>SPNIKIFSGSSHQDLSQKIADRLGLELGKVVTKKFSNQETCVEIGESVRGED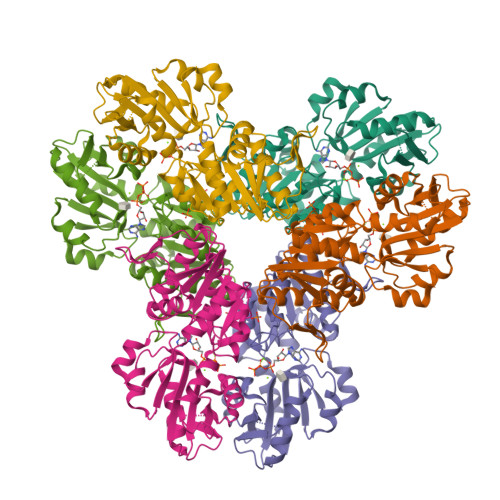VYIVQSGCGEINDNLMELLIMINACKIASASRVTAVIPCFPYARQDKKDKSRAPISAKLVANMLSVAGADHIITMDLHASQIQGFFDIPVDNLYAEPAVLKWIRENISEWRNCTIVSPDAGGAKRVTSIADRLNVDFALIHKERKKANEVDRMVLVGDVKDRVAILVDDMADTCGTICHAADKLLSAGATRVYAILTHGIFSGPAISRINNACFEAVVVTNTIPQEDKMKHCSKIQVIDISMILAEAIRRTHNGESVSYLFSHVPL[6x]Here, we study fold transition between distinct β-barrels by protein engineering and structural biology technique. Here, we discover that the previously reconstructed ancient DPBB sequence could also adopt a β-barrel fold named Double-Zeta β-barrel (DZBB), as a metamorphic protein. The DZBB fold is not found in any modern protein, although its structure shares similarities with RIFT and OB. Furthermore, the reconstructed OB fold could also be converted to the four-stranded SH3 fold by a simple circular permutation. Thus, these ancient β-barrel folds (DPBB, RIFT, OB, and SH3) could be readily interconverted by a few feasible mutations through the missing-link fold, DZBB, indicating their significantly close evolutionary relationships.

Design-1 exhibited the metamorphic property, adapting two different folds, DPBB and DZBB. Different ligand molecules probably induced the metamorphism in design-1. In the crystal structure of the DPBB-fold, two malonate ions bind to a positively charged pocket around the α1 helix, and are coordinated by Lys24, Arg27, and Lys33. Alternatively, in the crystal structure of design-1 with the DZBB fold, two additional residues, Arg21, and Arg18’ from the other chain, coordinate the two sulfates. The sulfate ions may attract these two additional residues in the folding process, and then stabilize the inverted β2-strand in the DZBB-fold. We also found that high concentrations of sulfate ion (≥1500 mM) increased ANS fluorescence. Its spectral pattern was slightly different compared to malonates, perhaps due to the difference in the DPBB- and DZBB-folds. The changes in the CD spectrum patterns depending on the sulfate ions were also observed. These experiments demonstrated that the small ions mediate the folding of design-1, and their types may lead to two different structures.

> KKVVARVAEARAEDVGKRVVRVDKAERAKVGVKVGDVVEVKKV>GSHMASAKAATKLADGKYNIAFTVWKGDKDESSRMNRYFESPATLTVKNGKQYVSFKVKDSTSIKSFQVEKDGQFVETTVLSENKKDNTRVVEFEVADLSKKLNGKVKINIPIINYNASYDIRFVFDGNSIK[2x]

B. anthracis, a Gram-positive pathogen that is a potential weapon for bioterrorism, secretes two hemophores (IsdX1 and IsdX2), that acquire heme from hemoglobin and promote bacterial growth in low-iron environments. The NEAT domain of IsdX1 is the only known NEAT domain to bind both heme and hemoglobin, as well as acquire heme from hemoglobin, thus making IsdX1 a useful model protein to study the relationship of these processes to one another. The structure consists of an immunoglobulin-like fold with eight β-strands arranged in two antiparallel β-sheets of a β-sandwich. The heme-binding pocket is enclosed primarily by a 310-helix (residues Arg-54 to Tyr-58) on one side of the heme and a long β-hairpin (β7–β8) on the other.

The heme bound form of IsdX1 was solved to 2.15 Å by molecular replacement using the structure of apo-IsdX1 as the search model. Heme-iron coordination is achieved through Tyr-136, which is conserved among all heme-binding NEAT domain proteins. The distance between the iron atom and the tyrosine oxygen ligand is 2.3 Å, which is typical for an Fe-O bond of NEAT domains. The coordination bond to iron is stabilized by the conserved residue Tyr-140, which forms a hydrogen bond with the phenolate oxygen of Tyr-136. The aromatic ring of Tyr-140 further stabilizes the pyrrole ring through π-stacking. The least solvent exposed heme propionate forms a hydrogen bond with the hydroxyl group of Ser-53, as well as the backbone nitrogen of Arg-54. Additionally, the side chain NH1 group of Arg-54 from chain A also hydrogen bonds to the least solvent exposed heme propionate, and also to the hydroxyl group of Ser-53. To accommodate the heme molecule, there is a shift in the residue sidechains of Arg-54 (2.5–2.8 Å), Arg-57 (7.3 Å), Tyr-58 (2.1 Å), Tyr-136 (1.6 Å) and Tyr-140 (2.6 Å), away from the center of the heme binding pocket. Met-55 in the holo structure has its side chain pointing into the interior of the protein and makes hydrophobic contacts with the heme pyrrole ring. Two heme molecules from adjacent subunits planar stack upon one another (inter-iron distance of 5.7 Å) and the crystallographic interface is further stabilized by two hydrogen-bonds; one from the NH2 group of Arg-54 from Chain A to the most solvent exposed heme propionate from Chain B and the second from the NH1 group from Arg-57 from Chain B to the hydroxyl group of Asn-135 on the adjacent molecule.>VVTAQWVPRVDIKEEVNHFVLYADLPGIDPSQIEVQMDKGILSIRGERKSESSTETERFSRIERRYG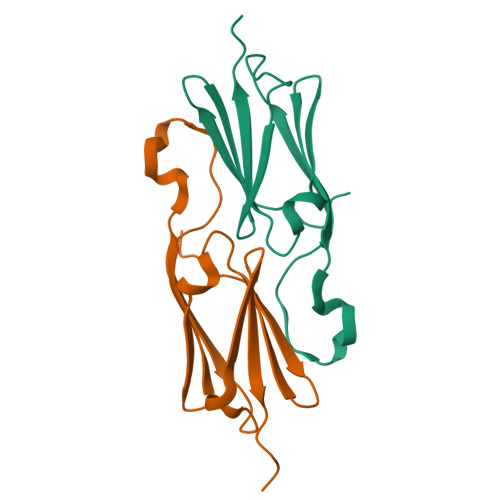SFHRRFALPDSADADGITAAGRNGVLEIRIPKRPAA[2x]>[4x]MKHHHHHHPMGATTQYTTLPSVLLIGPSGAGKTALLTLFERGPLLNPDGTSVGAADLKNPYRKPIVTSP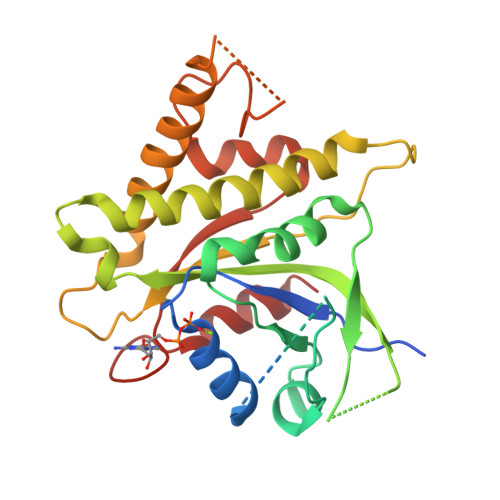VAQTHTSQVPTSVELAVGANEDGTPTSYKVDLDAAGATARKFLLIDTPGHPKLRGTTLQHLLNPSPSLTIIPTNAPNKKTSTDSHSDPYKSKLKAVIFLLDAAALADSDGDYLSQTASYLYDVLLSLQKRFHSRKNSRAPSSIPVLIAANKQDLFTAVPASLVKSRLEHELGRIRKTRQKGLLEASVTSEDEIRADDEEGWLGAVGSKEFKFEEMMEFDMEVEVMGGNVIGDGPGAERWWRWIGERI>MEVSPLQPVNENMQVNKIKKNEDAKKRLSVERIYQKKTQLEHILLRPDTYIGSVELVTQQMWVYDEDVGINYREVTFVPGLYKIFDEILVNAADNKQRDPKMSCIRVTIDPENNLISIWNNGKGIPVVEHKVEKMYVPALIFGQLLTSSNYDDDEKKVTGGRNGYGAKLCNIFSTKFTVETASREYKKMFKQTWMDNMGRAGEMELKPFNGEDYTCITFQPDLSKFKMQSLDKDIVALMVRRAYDIAGSTKDVKVFLNGNKLPVKGFRSYVDMYLKDKLDETGNSLKVIHEQVNHRWEVCLTMSEKGFQQISFVNSIATSKGGRHVDYVADQIVTKLVDVVKKKNKGGVAVKAHQVKNHMWIFVNALIENPTFDSQTKENMTLQPKSFGSTCQLSEKFIKAAIGCGIVESILNWVKFKAQVQLNKKCSAVKHNRIKGIPKLDDANDAGGRNSTECTLILTEGDSAKTLAVSGLGVVGRDKYGVFPLRGKILNVREASHKQIMENAEINNIIKIVGLQYKKNYEDEDSLKTLRYGKIMIMTDQDQDGSHIKGLLINFIHHNWPSLLRHRFLEEFITPIVKVSKNKQEMAFYSLPEFEEWKSSTPNHKKWKVKYYKGLGTSTSKEAKEYFADMKRHRIQFKYSGPEDDAAISLAFSKKQIDDRKEWLTNFMEDRRQRKLLGLPEDYLYGQTTTYLTYNDFINKELILFSNSDNERSIPSMVDGLKPGQRKVLFTCFKRNDKREVKVAQLAGSVAEMSSYHHGEMSLMMTIINLAQNFVGSNNLNLLQPIGQFGTRLHGGKDSASPRYIFTMLSSLARLLFPPKDDHTLKFLYDDNQRVEPEWYIPIIPMVLINGAEGIGTGWSCKIPNFDVREIVNNIRRLMDGEEPLPMLPSYKNFKGTIEELAPNQYVISGEVAILNSTTIEISELPVRTWTQTYKEQVLEPMLNGTEKTPPLITDYREYHTDTTVKFVVKMTEEKLAEAERVGLHKVFKLQTSLTCNSMVLFDHVGCLKKYDTVLDILRDFFELRLKYYGLRKEWLLGMLGAESAKLNNQARFILEKIDGKIIIENKPKKELIKVLIQRGYDSDPVKAWKEAQQKVPDEEENEESDNEKETEKSDSVTDSGPTFNYLLDMPLWYLTKEKKDELCRLRNEKEQE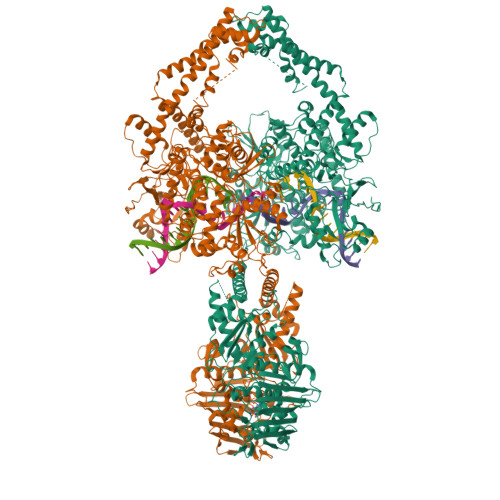LDTLKRKSPSDLWKEDLATFIEELEAVEAKEKQDEQVGLPGKGGKAKGKKTQMAEVLPSPRGQRVIPRITIEMKAEAEKKNKKKIKNENTEGSPQEDGVELEGLKQRLEKKQKREPGTKTKKQTTLAFKPIKKGKKRNPWSDSESDRSSDESNFDVPPRETEPRRAATKTKFTMDLDSDEDFSDFDEKTDDEDFVPSDASPPKTKTSPKLSNKELKPQKSVVSDLEADDVKGSVPLSSSPPATHFPDETEITNPVPKKNVTVKKTAAKSQSSTSTTGAKKRAAPKGTKRDPALNSGVSQKPDPAKTKNRRKRKPSTSDDSDSNFEKIVSKAVTSKKSKGESDDFHMDFDSAVAPRAKSVRAKKPIKYLEESDEDDLF[2x]> MIRNFHSLVKRVPRLALTPFFGFRTSMTLADKKLSTGEASVVLAEKIKGITQQNDITEYGTVISIGDGIARVFGLTKVQAGEMVEFKSGIRGMALNLETDNVGVVVLGNDRDIKEGDVVKRTGAIVDVPIGEAMCGRVFDALGNPIDGLGPLKTTQRARVEIKAPGIIPRQSVRQPMQTGIKCVDSLVPIGRGQRELIIGDRQTGKTAIAIDTILNQKEAFNTGDVKKQLYCIYVAVGQKRSTIANLVSILKQHDCMKFTIVVCATASDAAPLQFLAPYSGCAIGEFF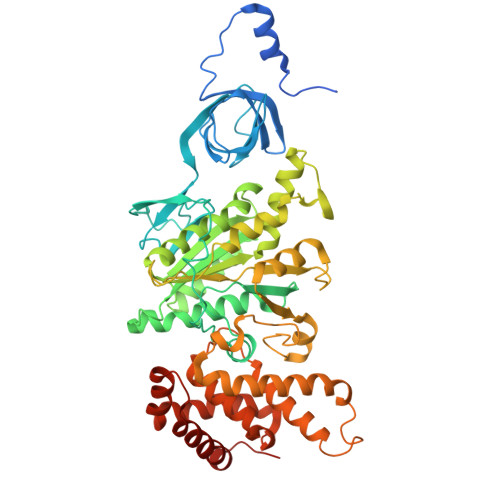RDNGKHALIIYDDLSKQAVAYRQMSLLLRRPPGREAYPGDVFYLHSRLLERAAKMNDSLGGGSLTALPVIETQAGDVSAYIPTNVISITDGQIFLETELFYKGIRPAINVGLSVSRVGSAAQIKAMKKIAGNLKLTLATYRELAAFSQFGSDLDAKTQQQLNTGERLVEMLKQNQYTPMKVEEQVCIIFAGVKGFLDALVTSEVLKFEKKFLEHVRTNHSALLKRIRDSGDLSEVDTNELNTIIPLFIQEGGFKLKAQ>[4x]GAMWHTHSEREKRVSNAVEFLLDSRVRRTPTSSKVH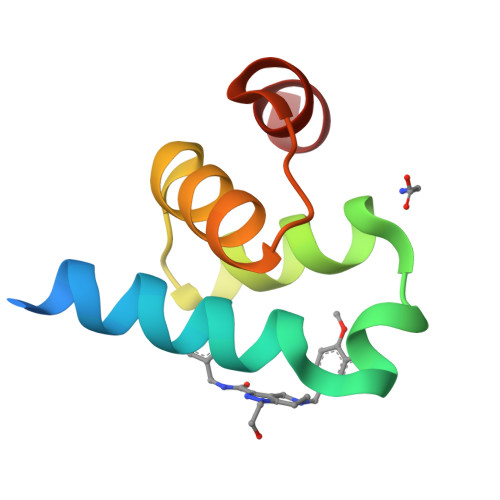FLKSKGLSAEEICEAFTKVGQPKTLNEIKRILS> TSIGLHGGRPRDIILDDAKGPLQNIVTWDEHSLFVHGERVVIFSGEVHPFRLPVPSLYLDVFHKIKALGFNTVSFYVDWALLEGKPGRFRADGIFSLEPFFEAATKAGIYLLARPGPYINAEVSGGGFPGWLQRVKGKLRTDAPDYLHATDNYVAHIASIIAKAQITNGGPVILYQPENEYSGAAEGVLFPNKPYMQYVIDQARNAGIIVPLINNDAFPGGTGAPGTGLGSVDIYGHDGYPLGFDCAHPSAWPDNGLPTTWRQDHLNISPSTPFSLVEFQGGAFDPFGGWGFEQCSALVNHEFERVFYKNNMAAGVTIFNIYMTFGGTNWGNLGHPGGYTSYDYGASIREDRRIDREKYSELKLQGQFLKVSPGYITATPENATQGVYSDSQNIVITPLLAKESGDFFVVRHANYSSTDTASYTVKLPTSAGDLTIPQLGGSLTLTGRDSKIHVTDYPVGKFTLLYSTAEIFTWNEFAEKTVLVLYGGAQELHEFAVKNPFGSSKTAKAKKIEGSN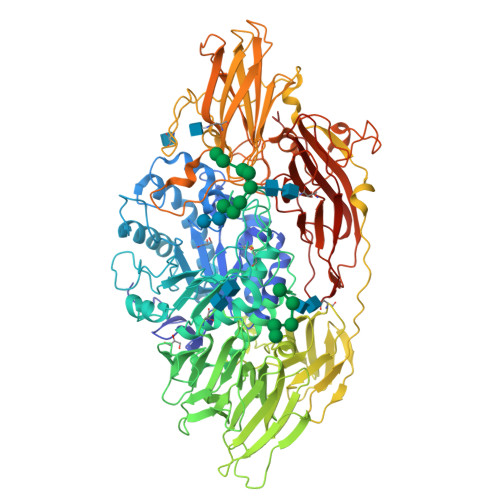VTIHTTSNLTVVLQWTASSARQVVQLGSLVIYMVDRNSAYNYWVPTLPGSGKQSAYGSSLMNPDSVIINGGYLIRSVAIKGNALSVQADFNVTTPLEIIGIPKGISKLAVNGKELGYSVSELGDWIAHPAIEIPHVQVPELTKLKWYKVDSLPEIRSNYDDSRWPLANLRTSNNTYAPLKTPVSLYGSDYGFHAGTLLFRGRFTARTARQQLFLSTQGGSAFASSVWLNDRFIGSFTGFDAASAANSSYTLDRLVRGRRYILTVVVDSTGLDENWTTGDDSMKAPRGILDYALTSSSGANVSISWKLTGNLGGEDYRDVFRGPLNEGGLFFERQGFHLPSPPLSDFTHGPSSSSSSSSPLDGIAHAGIAFYAAKLPLHLPAQEYDIPLSFVFDNATAAAPYRALLYVNGFQYGKYVSNIGPQTEFPVPEGILDYNGDNWIGVALWALESRGAKVPGLALKSKSPILTGRERVEVVKGPHFKKRHGAY> GSHMVSGKIVVIGSSTGGPRSLDMIIPNLPKNFPAPIVVVQHMPP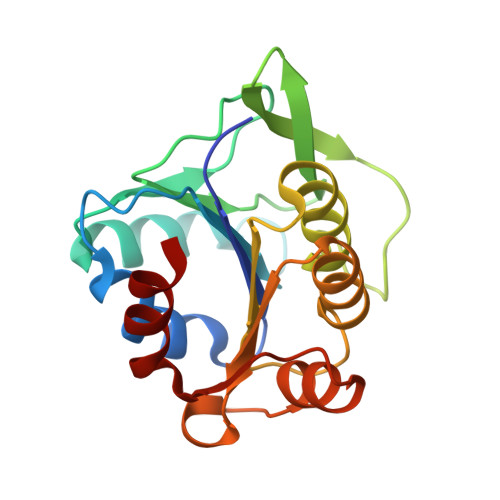GFTKSLAMRLDSTSELTVKEAEDGEEVKPGFVYIAPGDFHLGLKAQNGKVFFFLDKSDKINNVRPAVDFTLDKAAEIYKSKTIAVILTGMGKDGTKGAFKVKFYGGTVIAEDKETCVVFGMPKSVIEEGYADYVLPAYKIPEKLIELV8-(CYCLOHEXA-2,5-DIEN-1-YLIDENEAMINO)-1-(PIPERIDIN-4-YLMETHYL)-4,5-DIHYDRO-1H-PYRAZOLO[4,3-H]QUINAZOLINE-3-CARBOXAMIDE 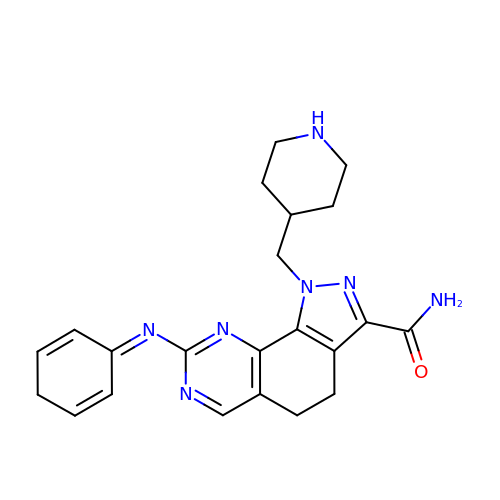| C22 H25 N7 O | NJZDNEMNAJYOMW-UHFFFAOYSA-N> GSTSARNHTEDNSTEYYDYE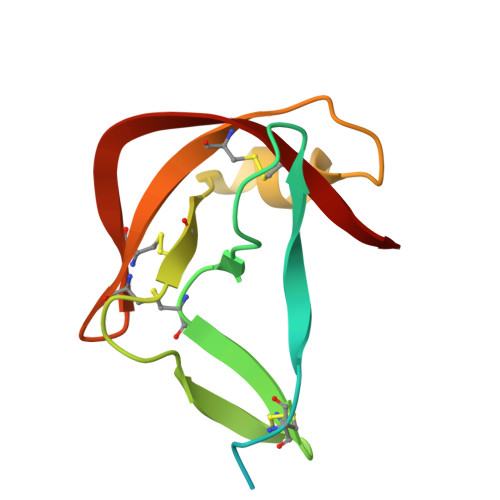EARSACPARHLNNTNGTVLKLLGCHYFCNGTLSTAPDGYPCYNLTAQQVRTLTTYPNTSCAVGVCMKGTCVKNGTMEQCFKTP> MAAPARDPPGYRYAAAMVPTGSILSTIEVASHRRLFDFFARVRSDENSLYDVEFDALLGSYCNTLSLVRFLELGLSVACVCTKFPELAYMNEGRVQFEVHQPLIARDGPHPVEQPVHNYMTKVIDRRALNAAFSLATEAIALLTGEALDGTGISLHRQLRAIQQLARNVQAVLGAFERGTADQMLHVLLEKAPPLALLLPMQRYLDNGRLATRVARATLVAELKRSFCDTSFFLGKAGHRREAIEAWLVDLTTATQPSVAVPRLTHADTRGRPVDGVLVTTAAIKQRLLQSFLKVEDTEADVPVTYGEMVLNGANLVTALVMGKAVRSLDDVGRHLLDMQEEQLEANRETLDELESAPQTTRVRADLVAIGDRLVFLEALEKRIYAATNVPYPLVGAMDLTFVLPLGLFNPAMERFAAHAGDLVPAPGHPEPRAFPPRQLFFWGKDHQVLRLSMENAVGTVCHPSLMNIDAAVGGVNHDPVEAANPYGAYVAAPAGPGADMQQRFLNAWRQRLAHGRVRWVAECQMTAEQFMQPDNANLALELHPAFDFFAGVADVELPGGEVPPAGPGAIQATWRVVNGNLPLALCPVAFRDARGLELGVGRHAMAPATIAAVRGAFEDRSYPAVFYLLQAAIHGSEHVFCALARLVTQCITSYWNNTRCAAFVNDYSLVSYIVTYLGGDLPEECMAVYRDLVAHVEALAQLVDDFTLPGPELGGQAQAELNHLMRDPALLPPLVWDCDGLMRHAALDRHRDCRIDAGGHEPVYAAACNVATADFNRNDGRLLHNTQARAADAADDRPHRPADWTVHHKIYYYVLVPAFSRGRCCTAGVRFDRVYATLQNMVVPEIAPGEECPSDPVTDPAHPLHPANLVANTVNAMFHNGRVVVDGPAMLTLQVLAHNMAERTTALLCSAAPDAGAN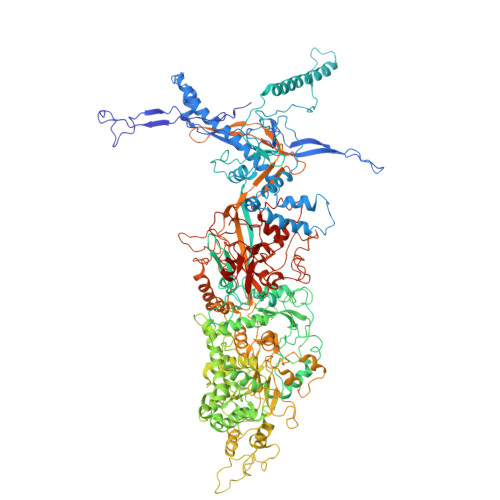TASTANMRIFDGALHAGVLLMAPQHLDHTIQNGEYFYVLPVHALFAGADHVANAPNFPPALRDLARHVPLVPPALGANYFSSIRQPVVQHARESAAGENALTYALMAGYFKMSPVALYHQLKTGLHPGFGFTVVRQDRFVTENVLFSERASEAYFLGQLQVARHETGGGVNFTLTQPRGNVDLGVGYTAVAATATVRNPVTDMGNLPQNFYLGRGAPPLLDNAAAVYLRNAVVAGNRLGPAQPLPVFGCAQVPRRAGMDHGQDAVCEFIATPVATDINYFRRPCNPRGRAAGGVYAGDKEGDVIALMYDHGQSDPARPFAATANPWASQRFSYGDLLYNGAYHLNGASPVLSPCFKFFTAADITAKHRCLERLIVETGSAVSTATAASDVQFKRPPGCRELVEDPCGLFQEAYPITCASDPALLRSARDGEAHARETHFTQYLIYDASPLKGLSL> TGVWEKTVNTEENVYATLGSDVNLTCQTQTVGFFVQMQWSKVTNKIDLIAVYHPQYGFYCAYGRPCESLVTFTETPENGSKWTLH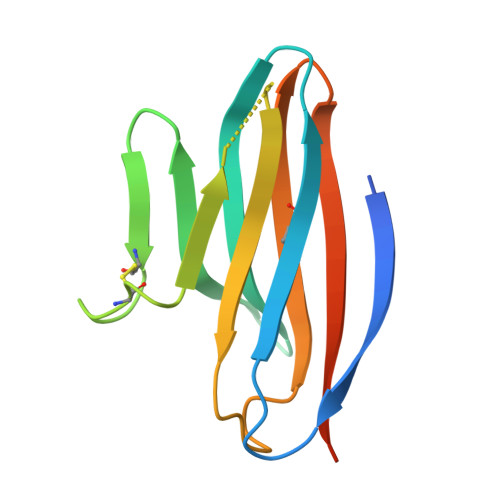LRNMSSSVSGRYECMLVLYPEGIQTKIYNLLIQTHGTHHHHHH One especially common junction element is the kink-turn (k-turn). k-turns are elements in double-stranded RNA that introduce a tight kink into the helical axis, with an included angle close to 50°. A standard k-turn comprises a three-nucleotide bulge followed by successive G•A and A•G trans G(sugar edge)•A(Hoogsteen edge) basepairs. k-turns are commonly-occurring motifs that introduce sharp kinks into duplex RNA, thereby facilitating tertiary contacts. Both the folding and conformation of k-turns are determined by their local sequence. k-turns fall into two conformational classes, called N3 and N1, that differ in the pattern of hydrogen bonding in the core. We show here that this is determined by the basepair adjacent to the critical G•A pairs.

We therefore decided to extend the study with a systematic structural analysis of HmKt-7 as a function of the 3b,3n sequence. This was performed in the constant environment of the SAM-I riboswitch, modified by replacing its natural k-turn by HmKt-7 with different 3b,3n sequences. However, we have shown previously that in other environments, this k-turn (abbreviated here to HmKt-7) adopts the N3 structure. Moreover, the various structures, with resolutions in the range 1.7 to 3.1 Å, have been determined in five different space groups, encompassing hexagonal, tetragonal and orthorhombic symmetries. Several include multiple molecules within the asymmetric unit and altogether there are 17 independent structures, all of which are unambiguously in the N3 conformation, and all in a closely similar conformation with a small RMSD values. 3b,3n = A•G is the only k-turn that folds in response to addition of metal ions to adopt the N3 conformation. For example, the 6 structures with 3b,3n = A•G all form trans-Hoogsteen-sugar edge basepairs.

> GGCUUAUCAAGAGAGGGGGAGUGACUGGCGCGAAGAACCCCGGCAACCAGAAAUGGUGCCAAUUCCUGCAGCGGAAACGUUGAAAGAUGAGCCG>AGAGAGATGGGTGCG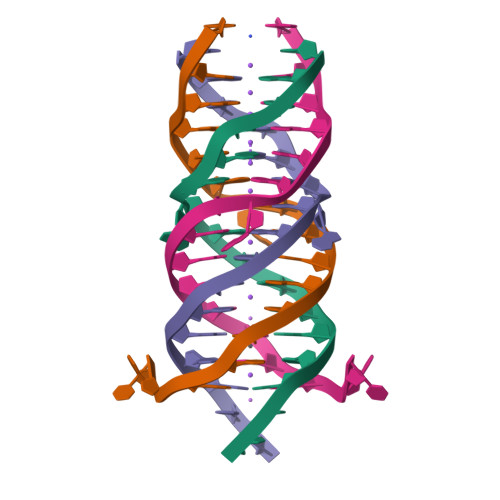TT[2x]>[10x]TPQNITDLCAEYHNTQIYTLND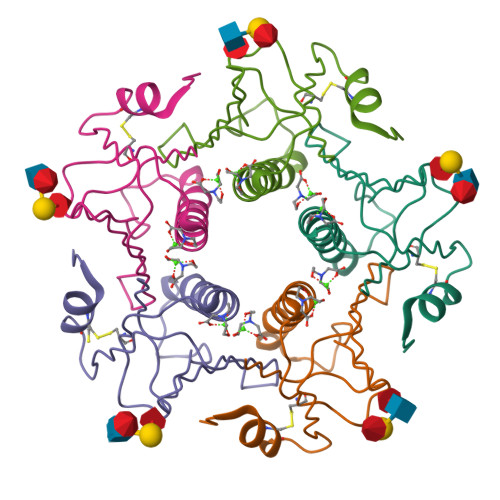KIFSYTESLAGKREMAIITFKNGAIFQVEVPGSQHIDSQKKAIERMKDTLRIAYLTEAKVEKLCVWNNKTPHAIAAISMAN> MRTFFVGGNWKANPKTVEEAEKLIEMLNGAKVEGNVEVVVAAPFYFLPTLQQKLRKDWKVSAENVFTKPNGA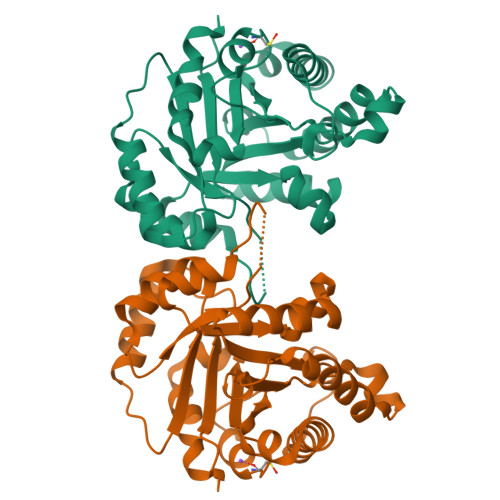FTGEVTVPMIKSFGIEWTILGHSERRDILKEDDEFLAAKAKFALENGMKIIYCCGEHLSEREAGKASEFVSAQIEKMIPAIPAGKWDDVVIAYEPIWAIGTGKVASTQDAQEMCKVIRDILAAKVGADIANKVRILYGGSVKPNNCNELAACPDVDGFLVGGASLEPGFINIVNSNVHSK>[2x]SNIGSGAPVVKEKLSPLHPDSPESEESYAEVPIESIQQFVQIYGIVRDNYVDEKSDDALFLQAIKGLVSGLDRYSRYLSAEEYRQLIQYTEG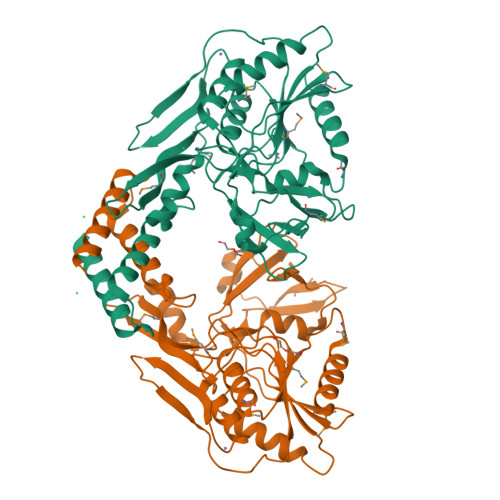DLASVDFVLSPESHVHKWMIRDLKTGSDSYKLGLRNGQTILKIDNQELKNLTHDQVLGLLYGSIGSTLQVQTEESNSPISLVRNKKIETDIEPVMLHNQVLVLKIRVFQQDTANEIKRLIEENSSSRLKAVLIDLRNNPGGLLSAAVESADLFLNHGIIVSTKSRSEGNQQFQALPGNDFQNIKVGILINHRSASAAEVFTAAMKEHQRAWVMGEKSYGKGVVQKLFPLPSGAALQMTVSHYYTPNGNMIEGQGIQPNQTYPLPPEMKEEVYLDRVADLLLKRK The collectin family of mammalian innate immune system proteins recognizes pathogens by the repeating pattern of carbohydrates on their surfaces and organizes their disposal through neutralization, agglutination, and opsonization while recruiting immune system cells for their destruction. Bovine serum conglutinin has been shown to bind, through the globular carbohydrate recognition domain (CRD), to specific carbohydrate structures on complement effector protein iC3b, which arises following activation and cleavage of complement component C3 (12). We present here high-resolution crystal structures with and without bound ligand of a recombinant fragment of the C-terminal carbohydrate recognition domain of conglutinin, the first crystal structures of a bovine collectin. The conglutinin CRD monomer has an overall topology similar to that of the known collectin structures.

A further structure was therefore determined, to a higher resolution of 0.97 Å, utilizing 2,4 methanepentanediol (MPD) as an alternative cryoprotectant. This structure did not show any extra electron density in the ligand-binding site, except for water molecules, and is therefore designated as the native structure. In the unliganded structure, the lack of electron density for the calcium ion at the Ca2 site is accompanied by a lack of electron density, or movement away from the site, for some of the side chains of the Ca2 coordinators. The second calcium ion Ca2 is not as tightly bound as Ca1 (as evidenced by higher B-factor compared with Ca1) and is not observed in the structure without bound ligand. This may be because of a number of interdependent factors including the loss of order of 318–323 in the calcium binding loop, loss of Ca2 coordination by Asn-318, the lack of an interaction between Asp-320 and ligand, and low calcium concentration in the crystallization buffer. In the unliganded and αGlcNAc-1-P–bound structures this Asn-318–Pro-324 loop is disordered. Within the structure without bound ligand there is some ill-defined electron density for the loop that could correspond to the ligand-bound loop, suggesting a small degree of order. However, it would not have been possible to discern the location of the loop without the prior knowledge of the position of the loop in the ligand-bound structures, supporting that the loop is mobile in the absence of ligand.

> KAVLFPDGQAVGEKIFKTAGAVKSYSDAEQLCREAKGQLASPRSSAENEAVTQMVRAQEKNAYLSMNDISTEGRFTYPTGEILVYSNWADGEPNNSDEGQPENCVEIFPDGKWNDVPCSKQLLVICEF> MGSSHHHHHHSQLEVLFQGPLGSGRPKKVPSAQTAYSVELARNLTWRRERKALLQEKKGLVNGNGTEMTSVQFPPPPNLAASAPRRSSLGFTLDLHRIQRDYIDLVPKHWHVISLSLSDGGHDLCITRLQAGQAPFVLRLPLERASSRDSSVDETDVFDFHTGRAELLEIIKEINRTCHDSRDMAAKGEREKWWAEREALDQRLKELLMNIEHVWLGGFRGVFSQHGRRPELLEKFRAMFEGVLDKHLPSRRQVGRGKKGK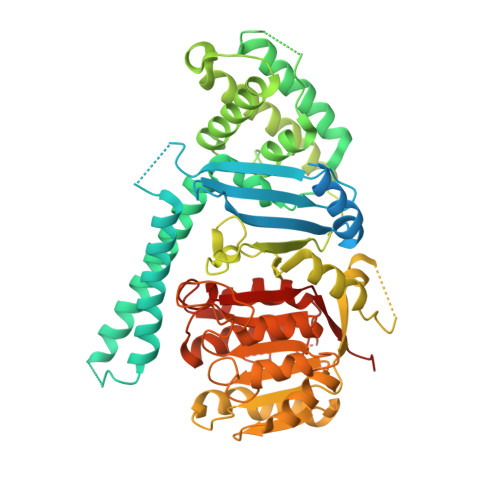GVAGQTKVVLDGNVLELFIGLGDATKSGADFDEELTDLLYFVVDILQFHGERNAYDEIDFDSMVVETMDALMAYHAEANAAPESDSHAHTILVLDKQLHVFPWESLPCLQGLAVSRIPSLACLRKLLLDRRRSSSQIQGEDSEEEDPRSAGHHAPLSGGTYILNPSSDLLSTQKTFESLFSTHLHSPNSWTRIISRPPTEPEFLSALTHSPILLYFGHGSGAQYIRSRNIRHLDHCRATVLLMGCSSAALTAKGEFEPSGPVWNYMLAGAPAVVGTLWDVTDRDIDRFAGGVLEGWGVLPEGCMGEKNGKKKAGRNGLSLVQAVAKARDRCRFRYVTAAAAVVYGIPVYVDVDGKSKD>[4x]MLSPKAATLAERSAGLAFSLYQAMAKDQAVENILLSPVVVASSLGLVSLGGKATTASQAKAVLSAEQLRDEEVHAGLGELLRSLSNSTARNVTWKLGSRLYGPS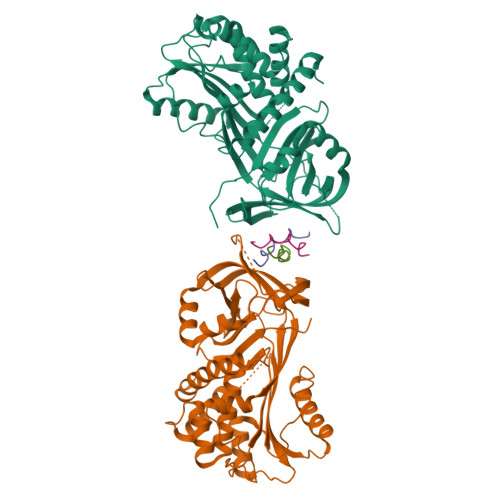SVSFAEDFVRSSKQHYNCEHSKINFRDKRSALQSINEWAAQTTDGKLPEVTKDVERTDGALLVNAMFFKPHWDEKFHHKMVDNRGFMVTRSYTVGVTMMHRTGLYNYYDDEKEKLQIVEMPLAHKLSSLIILMPHHVEPLERLEKLLTKEQLKIWMGKMQKKAVAISLPKGVVEVTHDLQKHLAGLGLTEAIDKNKADLSRMSGKKDLYLASVFHATAFEWDTEGNPFDQDIYGREELRSPKLFYADHPFIFLVRDTQSGSLLFIGRLVRPKGDKMRDELLEHHHHHH;>[6x]XPPGPPGPRGPPGPPX>[2x]MAATTENLPQLKSAVDGLTEMSESEKSGFISLVSRYLSGEAQHIEWSKIQTPTDEIVVPYEKMTPVSQDVAETKNLLDKLVVLKLNGGLGTTMGCTGPKSVIEVRDGLTFLDLIVIQIENLNNKYGCKVPLVLMNSFNTHDDTHKIVEKYTNSNVDIHTFNQSKYPRVVADEFVPWPSKGKTDK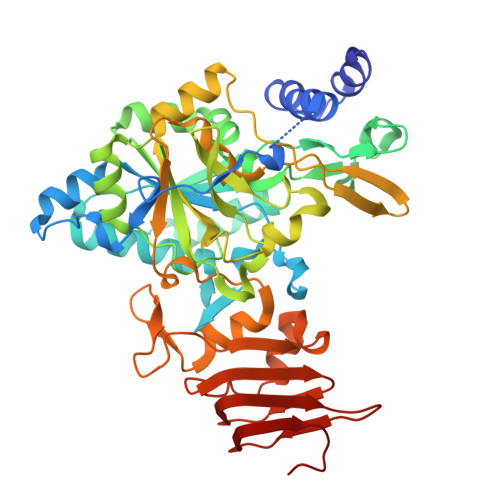EGWYPPGHGDVFPALMNSGKLDTFLSQGKEYVFVANSDNLGAIVDLTILKHLIQNKNEYCMEVTPKTLADVKGGTLISYEGKVQLLEIAQVPDEHVNEFKSIEKFKIFNTNNLWVNLKAIKKLVEADALKMEIIPNPKEVDGVKVLQLETAAGAAIRFFDNAIGVNVPRSRFLPVKASSDLLLVQSDLYTLVDGFVTRNKARTNPSNPSIELGPEFKKVATFLSRFKSIPSIVELDSLKVSGDVWFGSSIVLKGKVTVAAKSGVKLEIPDRAVVENKNINGPEDL> IRSFATHAQLPISIVNREDDAFLNP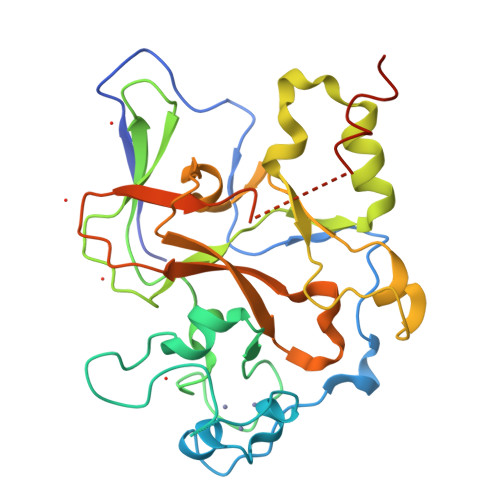NFRFIDHSIIGKNVPVADQSFRVGCSCASDEECMYSTCQCLDEMAPDSDEEADPYTRKKRFAYYSQGAKKGLLRDRVLQSQEPIYECHQGCACSKDCPNRVVERGRTVPLQIFRTKDRGWGVKCPVNIKRGQFVDRYLGEIITSEEADRRRAESTIARRKDVYLFALDKFSDPDSLDPLLAGQPLEVDGEYMSGPTRFINHSCDPNMAIFARVGDHADKHIHDLALFAIKDIPKGTELTFDYVNGLTGLESDAHDPSKISEMTKCLCGTAKCRGYLW>HMTDTHTGPTPADAVPAYPFSLPHALDLDPHYAELRRDEPVSRVRLPYGEGTAWLVTRMSDARIVLGDSRFSTAAATDPATPRMFPTPPEPDWVLAQDPPDHTRLRRLVGKAFTARRVEEMRPRVRSLVDSLLDDMVAHGSPADLVEFLAVPFPVAVICELLGVPLEDRDLFRTFSDAMLSSTRLTAAEIQRVQQDFMVYMDGLVAQRRDAPTEDLLGALALATDNDDHLTKGEIVNMGVSLLIAGHETSVNQITNLVHLLLTERKRYESLVADPALVPAAVEEMLRYTPLVSAGSFVRVATEDVELSTVTVRAGEPCVVHFASANRDEEVFDHADELDFHRERNPHIAFGHGAHHCI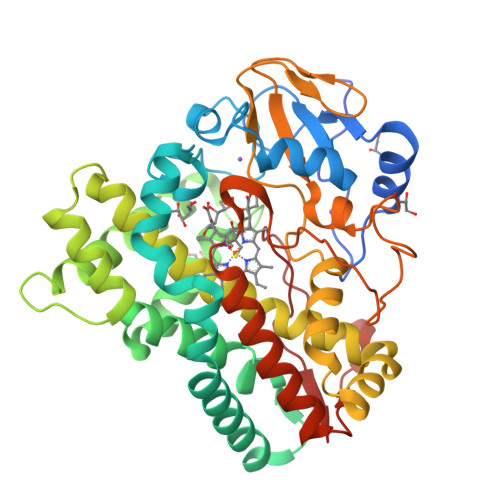GAQLGRLELQEALSALVRRFPTLDLAEPVAGLKWKQGMLIRGLERQIVSW[6x]>[4x]TTVMKFGGTSVGSGERIRHVAKIVTKRKKEDDDVVVVVSAMSEVTNALVEISQQALDVRDIAKVGDFIKFIREKHYKAIEEAIKSEEIKEEVKKIIDSRIEELEKVLIGVAYLGELT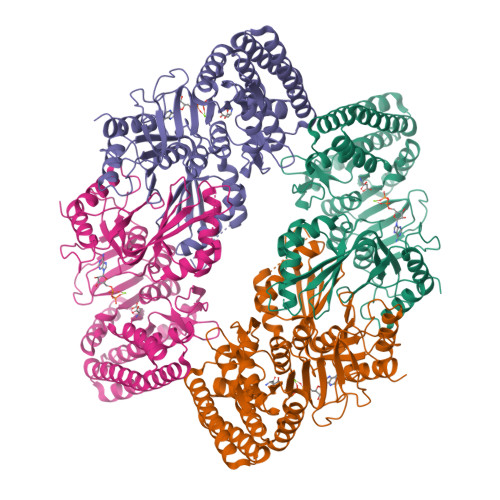PKSRDYILSFGERLSSPILSGAIRDLGEKSIALEGGEAGIITDNNFGSARVKRLEVKERLLPLLKEGIIPVVTGFIGTTEEGYITTLGRGGSDYSAALIGYGLDADIIEIWTDVSGVYTTDPRLVPTARRIPKLSYIEAMELAYFGAKVLHPRTIEPAMEKGIPILVKNTFEPESEGTLITNDMEMSDSIVKAISTIKNVALINIFGAGMVGVSGTAARIFKALGEEEVNVILISQGSSETNISLVVSEEDVDKALKALKREFGDFGKKSFLNNNLIRDVSVDKDVCVISVVGAGMRGAKGIAGKIFTAVSESGANIKMIAQGSSEVNISFVIDEKDLLNCVRKLHEKFIEK> QPIFLNVLEAIEPGVVCAGHDNNQPDSFAALLSSLNELGE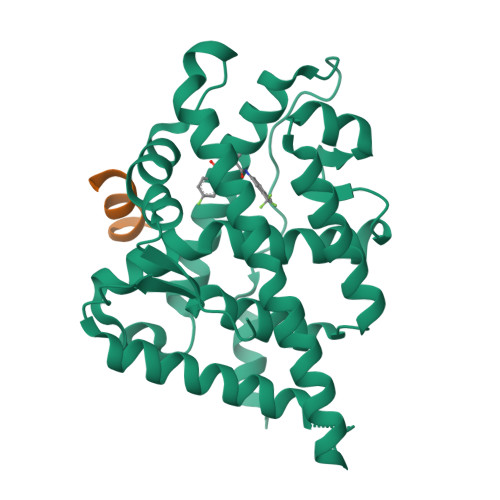RQLVHVVKWAKALPGFRNLHVDDQMAVIQYSLMGLMVFAMGWRSFTNVNSAMLYFAPDLVFNEYRMHKSRMYSQCVRMRHLSQEFGWLQITPQEFLCMKALLLFSIIPVDGLKNQKFFDELRMNYIKELDRIIACKRKNPTSCSRRFYQLTKLLDSVQPIARELHQFTFDLLIKSHMVSVDFPEMMAEIISVQVPKILSGKVKPIYFHTQ;> SDSAFSRLYTRS>[4x]MAHHHHHHMDKLIITGGNRLDGEIRISGAKNSALPILAATLLADTPVTVCNLPHLHDITTMIELFGRMGVQPIIDEKLNVEVDASSIKTLVAPYELVKTMRASILVLGPMLARFGEAEVALPGGCAIGSRPVDLHIRGLEAMGAQIEVEGGYIKAKAPAGGLRGGHFFFDTVSVTGTENLMMAAALANGRTVLQNAARE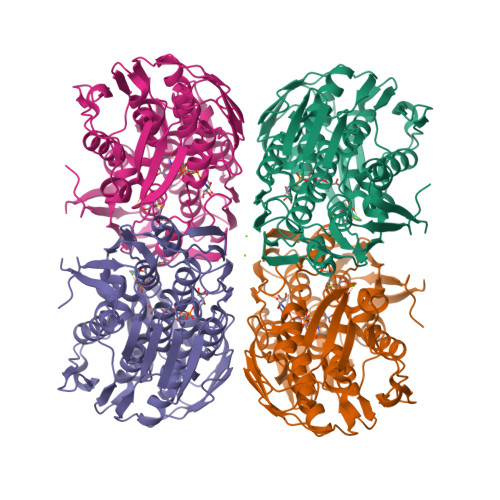PEVVDLANCLNAMGANVQGAGSDTIVIEGVKRLGGARYDVLPDRIETGTYLVAAAATGGRVKLKDTDPTILEAVLQKLEEAGAHISTGSNWIELDMKGNRPKAVNVRTAPYPAFPTDMQAQFISMNAVAEGTGAVIETVFENRFMHVYEMNRMGAQILVEGNTAIVTGVPKLKGAPVMATDLRASASLVIAGLVAEGDTLIDRIYHIDRGYECIEEKLQLLGAKIRRVPG>[5x]GVITAGFELKPPPYPLDALEPHMSRETLDYHWGKHHKTYVENLNKQILGTDLDALSLEEVVLLSYNKGNMLPAFNNAAQAWNHEFFWESIQPGGGGKPTGELLRLIERDFGSFEEFLERFKSAAASNFGSGWTWLAYKANRLDVANAVNPLPKEEDKKLVIVKTPNAVNPLVWDYSPLLTIDTWEHAYYLDFENRRAEYINTFMEKLVSWETVSTRLESAIARAVQREQEGTETEDEENPDDEVPEVYLDSDIDVSEVDAAALEHHHHHH

In Angiosperms, the plastid-encoded RNA polymerase (PEP) is a multimeric enzyme, essential for the proper expression of the plastid genome during chloroplast biogenesis. The PEP complex is composed of a prokaryotic-type core of four plastid-encoded subunits and 12 nuclear-encoded PEP-associated proteins (PAPs). PAP7 belongs to methyltransferases, PAP10 is a thioredoxin (TrxZ) while PAP4 (FSD3) and PAP9 (FSD2) are both iron superoxide dismutases (FeSOD). SODs are cellular defenses against superoxide by catalyzing the dismutation of superoxide into hydrogen peroxide according to the overall reaction: 2O2– + 2H+ → H2O2 + O2.

Five molecules of PAP9 are in the asymmetric unit. Four of them form two dimers. The fifth interacts with a molecule from another asymmetric unit to form also a dimer. The buried area calculated using PISA in the dimer interface is 1785 Å2. PAP9 is folded in two domains similar to those observed in FeSODs or MnSODs. The N-terminal domain extends from Gly1 to Gly93 and contains three α-helices. The C-terminal domain (Gly94–Gln229) displays an α/β fold with a three anti-parallel β-strands sandwiched by four α-helices and the N-terminal domain. No electron density is observed for residues from Arg141 to Glu155 and for the last 29 residues from Gly231 to Asp259 suggesting flexibility. The catalytic center is at the interface of the N- and C-terminal domains. The zinc ion is penta-coordinated by the His31, His83 side chains of the N-terminal domain, the Asp182, and His186 side chains from the α/β fold domain, and a water molecule supposed to mimic the position of the hydroxide ion.> GHSDVKQTIYEVNKYAKRSKLIEILSEQADGTIVFVETKRGADFLASFLSEKEFPTTSIHGDRLQSQREQALRDFKNGSMKVLIATSVASRGLDIKNIKHVINYDMPSKIDDYVHRIGRTGRVGNNGRATSFFDPEKDRAIAADLVKIL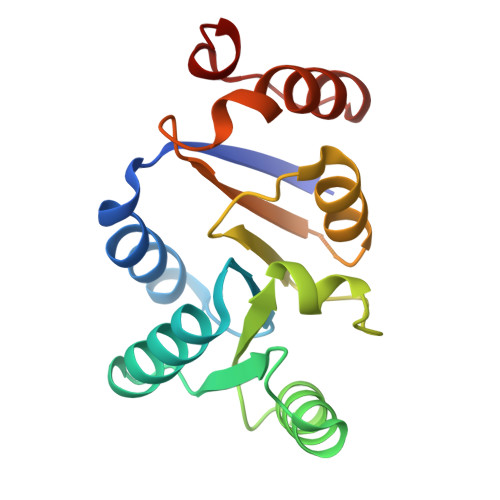EGSGQTVPDFLRTC> EVNXAE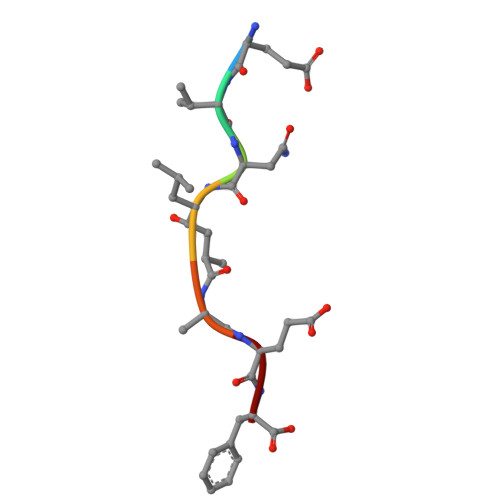F>MSPNRFLLCVCILGLIAGGAAKVQYALTIPALLKSGETQRACVNLIGYHQPLALSVVLEHQRVNISIFSEKVQPPHYFKCNKFMVPTVITNAPDFVTLSVSGGGEDIKDRKAVVIAPLNTICLIQMDKPVYKPGCKVRFRLISLNTMLLPISEKYTAVYLEDPSGSRIAQWQNQESVGGVVQLEFPLISDAAPGSYTITAEGESCESARQGFTVDEYILPRFSVIVDPPNTISILDDILTLNVSAIYTYGQPVPGSVTIKCCREASSYY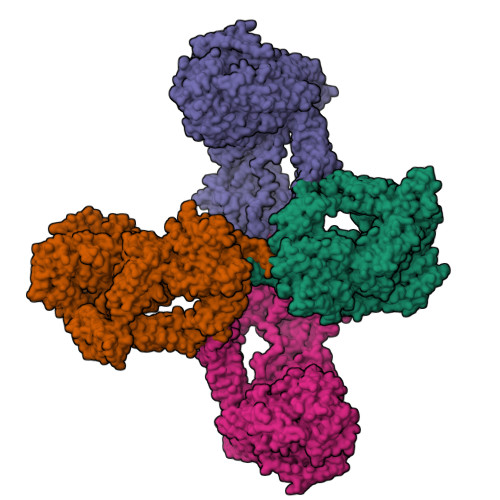GRKGNCFKGNRGICTNITGELGPDGAFYGVVSLLPFQMGQSGFQMSLGVALTVTEEGTGIQVTHQFFIMITSQLATLIFDYDALKEFYKRGIPYLVKVILTDANDNPMANEQVEVELAGKTIGAVLTDKEGRAEYAIDTSSFVQENFTVVVSYENPHQCYYTEWEGPDFPTAQHFVMRFYSETGSFLDIQGSSVELNCGQVHNISVRYILSLDGMGEGATTATFYYLAMSRAKIVQHGQRDVHLNQSKSGLFNIGLNVTSDLAPGAELIVYCILDLELIADTISLDIEKCFQNQVSLSFSDDLGPTASNVSLNLSAAPGSLCGVKVIDSSLLLINPYESLSASGVYYSIPYLSLFGYNYGGFNLEEPEPPCEDPNTVIFCKGRYYLPVSSSTEGDTYQNLRRVGLVLGTSSKIRKPVVCGMEAKFSVPRKSSGESDFGSSLSNGHVETLRKNFSETFLWRLVSVDSEGQNTITETVPDTITKWQGSMFCVSEKEGFGITKYSANFTSFLPFFVELSLPYSLTREEILVMKAFVSNYLEECIKIIVTLQPSADFEVIPQDVKQDQCICSGGRSSYSWNIIASSLGRISFIVSAETTHIGASCDGPSDQSQSTRKDTVIQTILVQPEGIRKEETSSNLVCVEDSNVEMPINLTLPENIVQGSASAFVTFVGDVLGLPLSNLQNLLQMPYGCGEQNLARMAPIPYVLEYLNNTNQLTDELLQTAVQFLNEGYYRQLRYKLPSGAYDAFWSSPSDGSSWLSAYTFKTFEKAKKYIYVDGKIQQQTLLYLQTSQKLDNGCFKAEGNLFMRQCGQERDLCFTAYLAIALLESNYSSGMTLLDDALGCLEAAMSSASTLYFKSYTVYVFTLVQNWEIRNTLLNELKSKVVSERGTLHWEREDKLGQEGIPLYYPNYSPAEVEITAYMLLSIAKGSDPTHDDLTYMAQISVWLIQQQNSYGGFRSTQDTVVALQALAFYAQLLFKSNAHHNVFLRSEYGDVGQLNLSEHNRLVVQRLQLPEVSGNYSISINGTGCCLVQSTIRYNIPVPKENSAFYVAADSVSKNCLNGVAYTITITVSVSYRGLRNETNMVIIDIQMLSGYQADYPSLRQLENSQQVSKTEEQDNHVFLYLNAVPLKTIQLSFKVLIGSRVLNVKSASVYVYDYYETGENGFASYSQPC[4x]> MNNVLNSGRTTICDAYNVVAHDPFSFEHK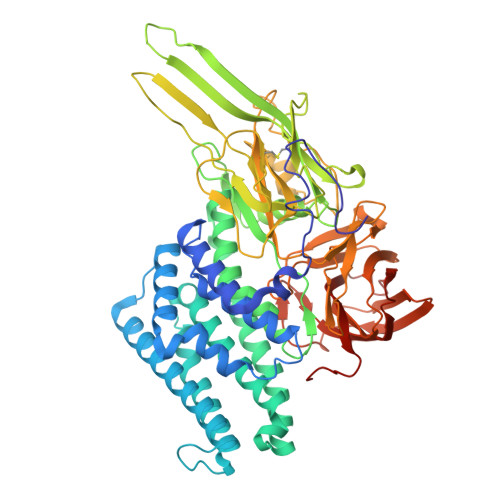SLDTIQKEWMEWKRTDHSLYVAPVVGTVSSFLLKKVGSLIGKRILSELWGIIFPSGSTNLMQDILRETEQFLNQRLNTDTLARVNAELIGLQANIREFNQQVDNFLNPTQNPVPLSITSSVNTMQQLFLNRLPQFQIQGYQLLLLPLFAQAANMHLSFIRDVILNADEWGISAATLRTYRDYLRNYTRDYSNYCINTYQTAFRGLNTRLHDMLEFRTYMFLNVFEYVSIWSLFKYQSLMVSSGANLYASGSGPQQTQSFTAQNWPFLYSLFQVNSNYILSGISGTRLSITFPNIGGLPGSTTTHSLNSARVNYSGGVSSGLIGATNLNHNFNCSTVLPPLSTPFVRSWLDSGTDREGVATSTNWQTESFQTTLSLRCGAFSARGNSNYFPDYFIRNISGVPLVIRNEDLTRPLHYNQIRNIESPSGTPGGARAYLVSVHNRKNNIYAANENGTMIHLAPEDYTGFTISPIHATQVNNQTRTFISEKFGNQGDSLRFEQSNTTARYTLRGNGNSYNLYLRVSSIGNSTIRVTINGRVYTVSNVNTTTNNDGVNDNGARFSDINIGNIVASDNTNVTLDINVTLNSGTPFDLMNIMFVPTNLPPLY>[2x]GSQIPASEQ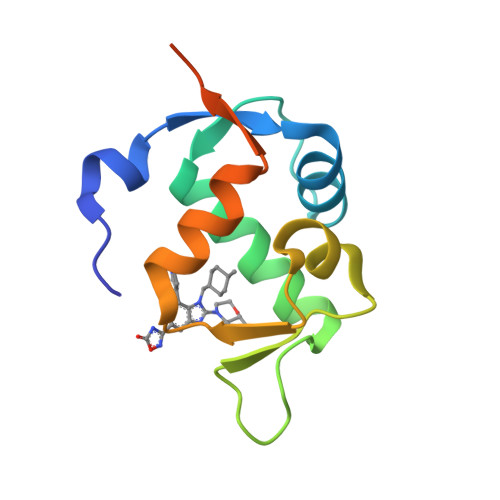ETLVRPKPLLLKLLKSVGAQKDTYTMKEVLFYLGQYIMTKRLYDEKQQHIVYCSNDLLGDLFGVPSFSVKEHRKIYTMIYRNLVVVNQQESSDSGTSVSEN>MHHHHHHITSLYKKAGFMRKNFLNIEELKRFLNGQTVVSIQPVTGSPLDKTDFIVAMAIAVEQAGAKALRIEGVSNVAAVSAAVTIPIIGIVKRDLPDSPVRITPFVSDVDGLANAGATVIAFDATNRTRPESRERIAQAIKNTGCFAMADCSTFEDGLWANSQGVEIVGSTLSGYVGDIEPTVPDFQLVKAFSEAGFFTMAEGRYNTPELAAKAIESGAVA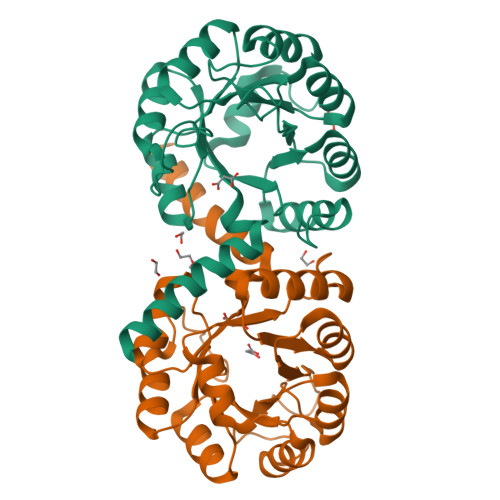VTVGSALTRLEVVTQWFNNATQAAGERKCAH[2x]>MTNLQDQTQQIVPFIRSLLMPTTGPASIPDDTLEKHTLRSETSTYNLTVGDTGSGLIVFFPGFPGSIVGAHYTLQGNGNYKFDQMLLTAQNLPASYNYCRLVSRSLTVRSSTLPGGVYALNGTINAVTFQGSLSELTDVSYNGLMSATANINDKIGNVLVGEGVTVLSLPTSYDLGYVRLGDPIPAIGLDPKMVATCDSSDRPRVYTITAADDYQFSSQYQPGGVTITLFSANIDAITSLSVGGELVFRTSVHGLVLGVTIYLIGFDGTTVITRAVAANNGLTTGTDNLMPFNL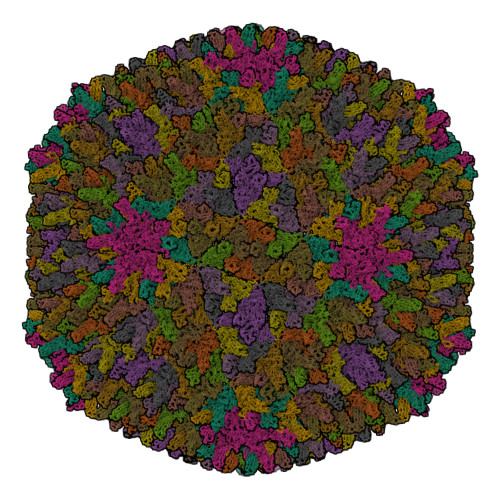VIPTNEITQPITSIKLEIVTSKSGGQAGDQMSWSARGSLAVTIHGGNYPGALRPVTLVAYERVATGSVVTVAGVSNFELIPNPELAKNLVTEYGRFDPGAMNYTKLILSERDRLGIKTVWPTREYTDFREYFMEVADLNSPLKIAGA[13x]Coxsackievirus A10 (CVA10), belonging to the human type-A Enterovirus (HEV-A) subgroup, used to be associated mainly with herpangina, but in recent years has been increasingly reported to co-circulate with other members of the genus such as enterovirus 71 (EV71), CVA16 and CVA6 causing hand, foot, and mouth disease (HFMD) outbreaks in Asia, Europe, and North America2,3. Like most members of the picornavirus family, HEV-As comprise 60 copies of viral proteins VP1, VP2, VP3, and VP4 arranged in pseudo T = 3 symmetry, encasing a positive-sense single-stranded RNA genome. Intriguingly, although CVA10 shares ~69% amino-acid sequence identity with EV71 and CVA16, it utilizes a different receptor, KREMEN1, for entry into host cells, suggesting CVA10 might differ in its mode of entry into host cells or perhaps even in its local structural features that are involved in receptor recognition. Here, we provide models for CVA10 mature virus, empty- and A-particles at atomic resolution, and establish details of the events covering a staged exit of the VP1 N-terminus and ordered structural reorganizations of VP1 GH, VP2 A2B and VP3 GH loops and alterations of viral genome structure as well as genome–capsid interactions during the uncoating.

Here, we report the atomic model of CVA10 mature virus built from a 3.0-Å resolution cryo-EM map. Except for a few disordered residues in VP4 (residues 1–18) and VP2 (residues 1–9), the mature CVA10 is well ordered. The capsid proteins VP1, VP2, and VP3 adopt the classical eight-stranded anti-parallel β-barrel configuration and follow the expected pseudo T = 3 symmetry, where VP1 surrounds the fivefold axes and VP2 and VP3 alternate about the two- and threefold axes. When compared to the structures of EV71 and CVA16, the external surface of CVA10 exhibits five additional continuous and “star-shaped” dense protrusions surrounding the fivefold axes. These arise as a result of the loops at the fivefold axes, in particular the VP1 BC loop, which assumes a raised configuration. However, compared to EV71 and CVA16, the raised conformation of the VP1 BC loop forming the north wall of the canyon and the refolding of the VP1 GH loop (front part of the south wall) from a short helix to a more extended loop moving away from the “star-protrusion” broaden the front portion of the canyon of CVA10. In contrast, the VP2 EF loop (back part of the south wall) of CVA10 bears a distinct conformation and moves closer towards the “star-protrusion”, narrowing the back portion of the canyon. It is quite likely that these conformational changes of the canyon and neighboring microenvironments, including VP3 BC loop, implicated in receptor and neutralizing monoclonal antibody binding, together with the alteration in electrostatic properties, determine the specificity of CVA10 for KREMEN1 during host cell entry and specify the antigenic sites of CVA10.

> GDPVEDIIHDALGSTARRAISSATNVESAANTTPSSHRLETGRVPALQAAETGATSNATDENMIETRCVVNRNGVLETTINHFFSRSGLVGVVNLTDGGTDTTGYVTWDIDIMGFVQLRRKCEMFTYMRFNAEFTFVTTTKNGEARPYMLQYMYVPPGAPKPTGRDAFQWQTATNPSVFVKLTDPPAQVSVPFMSPASAYQWFYDGYPTFGQHPETSNTTYGLCPNNMMGTFAVRVVSREASQLKLQTRVYMKLKHVRAWVPRPIRSQPYLLKNFPNYDSSKITNSARDRSSIKQAN;> SPSVEACGYSDRVAQLTVGNSSITTQEAANIVLAYGEWPEYCPDTDATAVDKPTRPDVSVNRFYTLDSKMWQENSTGWYWKFPDVLNKTGVFGQNAQFHYLYRSGFCLHVQCNASKFHQGALLVAVIPEFVIAGRGSNTKPNEAPHPGFTTTFPGTTGATFHDPYVLDSGVPLSQALIYPHQWINLRTNNCATVIVPYINAVPFDSAINHSNFGLIVIPVSPLKYSSGATTAIPITITIAPLNSEFGGLRQAVSQ;> GIPAELRPGTNQFLTTDDDTAAPILPGFTPTPTIHIPGEVHSLLELCRVETILEVNNTTEATGLTRLLIPVSSQNKADELCAAFMVDPGRIGPWQSTLVGQICRYYTQWSGSLKVTFMFTGSFMATGKMLVAYSPPGSAQPANRETAMLGTHVIWDFGLQSSVSLVIPWISNTHFRTAKTGGNYDYYTAGVVTLWYQTNYVVPPETPGEAYIIAMGADLYKFTLKICKDTDEVTQQAVLQ;> MGAQVSTQKSGSHETGNVATGGSTINFTNINYYKDSYAASATRQDFTQDPKKFTQPVLDSIRELSAPLN> MSHHHHHHSGLVPRGSMAWHLGIRSQSRPNDIMAEVCRAIKQLDYEWKVVNPYYLRVRRKNPVTSTFSKMSLQLYQVDSRTYLLDFRSIDDEITEAKSGTATPQRSGSISNYRSCQRSDSD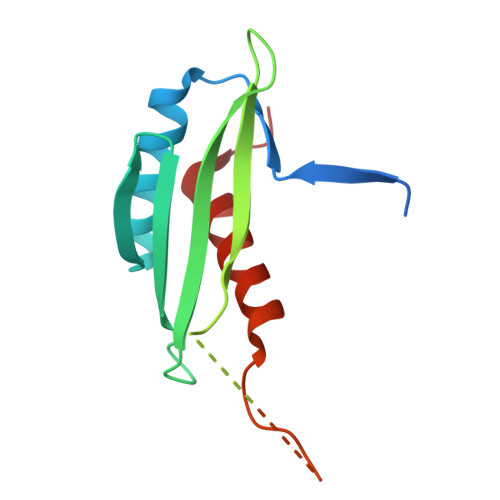AEAQGKPSEVSLTSSVTSLDSSPVDVAPRPGSHTIEFFEMCANLIKNSCTVN> GPGTRRFERDPTIPPDSIKVYSRTLFLGGITRSVREPVLRSMFERFGSVQSLILNHNYRHGFLKMFRRDAAEKAQVAMENVPFADTTIRTKWGVGFGPRECSDFSTGISVIPIRLLTD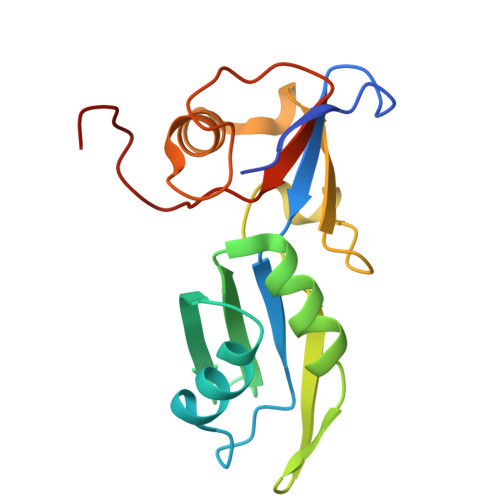ADRTWLVTAEYGGTGGLPITPGIALDEPDIEIGLGISSK>MAWPKVQPEVNIGVVGHVDHGKTTLVQAITGIWTSKHSEELKRGMTIKLGYAETNIGVCESCKKPEAYVTEPSCKSCGSDDEPKFLRRISFIDAPGHEVLMATMLSGAALMDGAILVVAANEPFPQPQTREHFVALGIIGVKNLIIVQNKVDVVSKEEALSQYRQIKQFTKGTWAENVPIIPVSALHKINIDSLIEGIEEYIKTPYRDLSQKPVMLVIRSFDVNKPGTQFNELKGGVIGGSIIQGLFKVDQEIKVLPGLRVEKQGKVSYEPIFTKISSIRFGDEEFKEAKPGGLVAIGTYLDPSLTKADNLLGSIITLADAEVPVLWNIRIKYNLLERVVGAKEMLKVDPIRAKETLMLSVGSSTT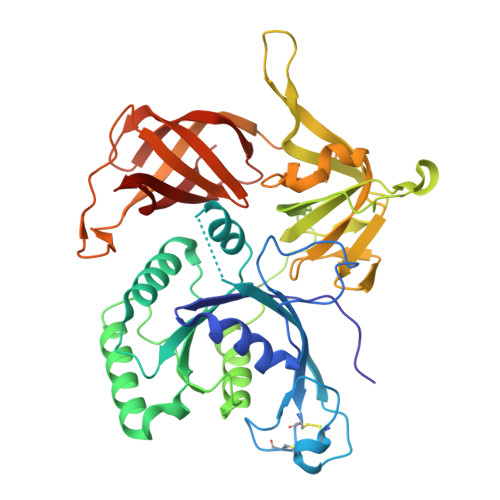LGIVTSVKKDEIEVELRRPVAVWSNNIRTVISRQIAGRWRMIGWGLVEI[2x]>[2x]MTTERQRTAPGLLAALHQARSRFGRPLDAQALAELSTAFSLPPGEIAATASFYHFFQTPPARYQIHFVDHVVDHHAGVAALCNHLCAAFAIQPGQRTADARLFVGWTACAGLSDQAPAALINGRPMPRLDAARIDALIEKIQAQIPMDQWPTEWFAVTNAIHRHGPLLTWLDTTPAEAVFEHPTAHDPDAILQAVTDAGLRGRGGAGFPTATKWRFCRENADPERFLICNADEGEPGTFKDRVLLTRYPEHLFAGMILAARAIGADKAILYLRYEYQYLLPQLEAARERIASAQATVPQAERVTLEIALGAGAYVCGEESALIESLEGKPGRPRVRPPYPVTQGYLGHPTVVNNVETLVAVAAIVGNGAAWWRALGTPDSSGPKLFCVSGDVAQPGLYEFPYGVALGDVVTAARPLGTRYAVQVSGPSGTLLPATPEQLARPLAFEALPCNGTVMVFDVRRDPVAIVHHFARFFAHESCGFCTPCRVGTQLIAKTFEKIAAGYATRFDLERLAPALEAMRLASNCGFGLSAGNPVRDLIAHFRQQLEAQLQPHDFIPAFSLDAELAATRRLTGRDDPHAHLAQFEQPEVTR;>[2x]MRPTTPPFASETFTLDEESIPFVPGQTVLEAALAAGRYIPHLCWHPEMGNHGSCRLCVVEANGRIQASCALPAQPGLQVVSKSETLTRVR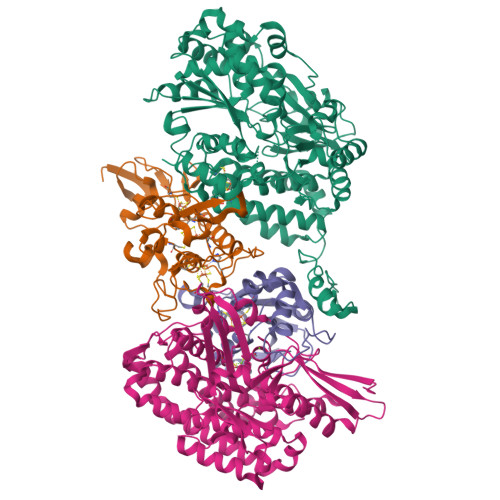RTLLEMLFAEGNHFCPGCEKSGDCLLQALAYAHGMTASHFDPFYPQRRIDASHPDLWLDPNRCILCGLCVRASLAEGKEALVIGGRGIASRLLATSASGRLGDTALAATDRAARICPVGALNFKAAGFTTPIGKRRFDHRPPEAMSDKERYT;>MTSAAPSAMPPRKIRIATASLAGCFGCHMSFADIDTRLLALAEWVTFDRSPLTDWKTVGECDIALIEGGVCNAENVEVLRAYRRAARILVAVGACAINGGLPAQRNQHRVERLLTQVFEADRHLAPGSRVPNDPELPLLLEHVHPIHEIVRVDYYLPGCPPTAEVIWTFLTDLLVGREPHFPYPTLRYD[2x];>[2x]MTQHAPQAVSPRPSLPANATRRVAIDPLSRVEGHGKVTIWLDDDGQVVEARLHIVEFRGFEAFIVGRPYWEAPVVVQRLCGICPVSHHLAAAKALDRLVGVTQLPPTAEKMRRLMHYGQVLQSHALHFFYLAAPDLLLGFSADPAQRNVFGLAAQKRELARQGILVRQFGQECIEATAGKRIHGTSAVPGGIHKNLSRRERMALLSRAPEIRSWCEAAVALIERLFTEHAPFFAQFGSFQTKTFSLVAADGSLDLYDGTFRVKEANGAILIDHYDPNDYDQLLVEAVRPWSYMKFPYLKAYGEPDGFYRVGPSARLINCDRLTTARAEAARQRFLTFDQGTVAHSTLGYHWARLIEMLHCAELIEALLTDADLEGGELRARGQRQHRGVGVIEAPRGTLIHHYEVGDDDLITYCNLIVSTTHNNAVMNQAVTTAAKAFLSGVTLTEALLNHIEVAVRAFDPCLSCATH>[4x]MQNITYSWFVQGMIKATTDAWLKGWDERNGGNLTLRLDDADIAPYHDNFHQQPRYIPLSQPMPLLANTPFIVTGSGKFFRNVQWDPAANLGIVKVDSDGAGYHILWGLTNEAVPTSELPAHFLSHCERIKATNGKDRVIMHCHATNLIALTYVLENDTAVFTRQLWEGSTECLVVFPDGVGILPWMVPGTDAIGQATA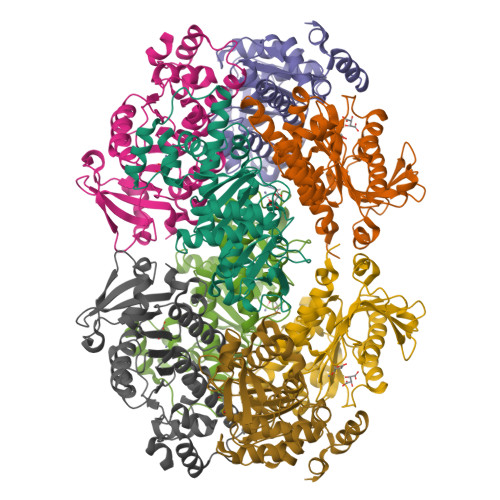QEMQKHSLVLWPFHGVFGSGPTLDETFGLIDTAEKSAQVLVKVYSMGGMKQTISREELIALGKRFGVTPLASALAL> MPRRSARKAQSAIASPADTNVVPAKDAPTTNSPPSTTSPNQAAADANQQQAGIVSSQSGPNAVGDSAPSSSVNNDGDIITRPTSDSIAAVANATKPAAVVSDPQSMKVTPIVNPSSYVCNVCNARFSTMSALSEHLRSDHRDDASTLLATPMINNAIRSFLTAWDDIRILSPDVSSKSLSAYLDSAVANGPELIIEDTGLCTSFMLLDNIPSAHLTKELIGFTWFMQMYQMTPPLPEGAVNRIVCMTNWASLGDEGRGLEVRLPPPTDSSVHAYKTVLSRGYIDNAQFNPLALRSNVLLMLLQFTLSNLKINKSSTFTSDVTTITSGRMIRAFEGRPELLALAYPGRAVLPTQTKNAQFLSTAIADRIGRLDRANLIGGEVSAMVECMELCDALTLHIRETYIMLLRSMHQDPTQIVQIVNECANNLLNSTIPISLRPTILCPWFASSEDLRLQQVMHLVNISSNTAAALPLVEALSTLLRSVTPLVLDPTVLTNAITTISESTTQTISPISEILRLLQPMGNDYAAFWKCIASWAYNGLVTTVLSEDAFPDSSQSITHLPSMWKCLFLTLAGPMTSDPHSPVKVFMALANLLAQPEPIAIGVPGMHQTTPASQFSHPGVWPPGFLNPQLINPQQAPLLRAFAEHIRANWPQPSEFGYGSTLQGSANLFIPSNRMVYPWPNQPLPRLTVAPTYDSAMSNWISTTIAFFIRVVNSVNMTATVNDLTRRTMTGVMTAMRQVKTMTPFYIQHMCPTELSVLASVTVTPPFQVPFTRLVQNDVITNVLVARVDPAQRGDAAVDIRATHATFAAALPVDPAAIVVAMLCGQTETNLIPSHHYGKAFAPLFASNAMFTRNQRAVITREAFVCARSAVAQCQDAGFLVPRPLDALRQFDVTSAAAAEIMHAVNDAFKTAFDLDGALLDGLALYGDPRIADLSAAYLQYGGNVVREHVPPGPSHIHRALQQVESTFMAEMNLFNVARGNLYLVQTATNGNWSPMAPVAAPPFVRGGPNVRVVGRFGTIVPRPNGLEPQLIDDGNVPRDIAGDWVYPSDVLQVSVAVFRDYVWPMVKAGRTRVLVELGHYVYTLHYYDPQISLDEAPILEEWLSKINPAGIPPVPFCIPIPQVY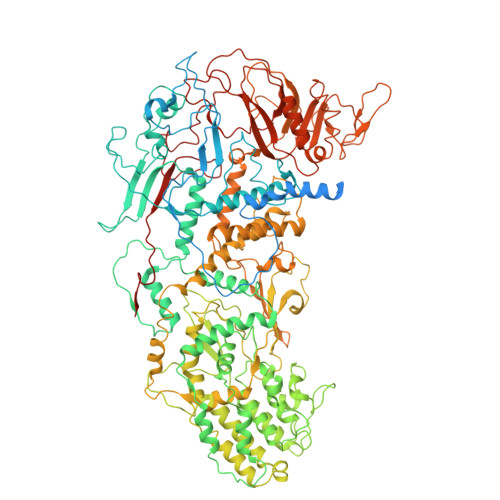PCITARRVHYAFTSENNNDSLFSTNAASIDTAFGENAAVSPLRWPGLVDPNYRVGTNDLPNRITLYNSLYRYNFTYPTLDGIMYVRSAT>[4x]MGSSHHH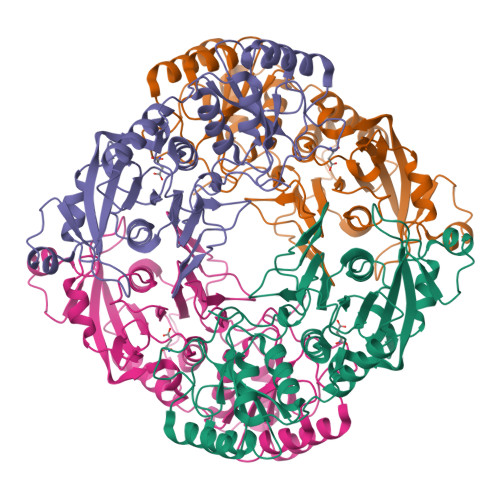HHHSSGGNENLYFQGHMARASGSERHLLLIYTGGTLGMQSKGGVLVPGPGLVTLLRTLPMFHDKEFAQAQGLPDHALALPPASHGPRVLYTVLECQPLLDSSDMTIDDWIRIAKIIERHYEQYQGFVVIHGTDTMASGASMLSFMLENLHKPVILTGAQVPIRVLWNDARENLLGALLVAGQYIIPEVCLFMNSQLFRGNRVTKVDSQKFEAFCSPNLSPLATVGADVTIAWDLVRKVKWKDPLVVHSNMEHDVALLRLYPGIPASLVRAFLQPPLKGVVLETFGSGNGPSKPDLLQELRAAAQRGLIMVNCSQCLRGSVTPGYATSLAGANIVSGLDMTSEAALAKLSYVLGLPELSLERRQELLAKDLRGEMTLPT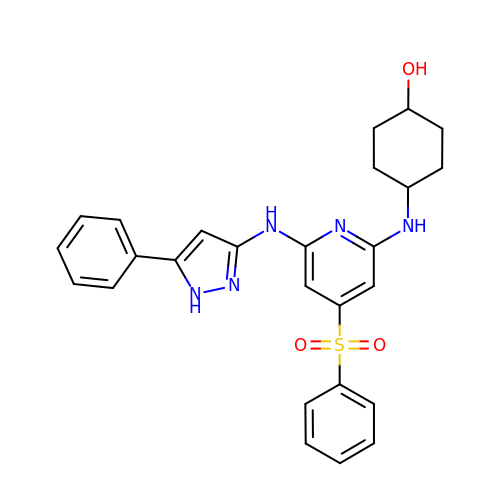trans-4-({6-[(5-phenyl-1H-pyrazol-3-yl)amino]-4-(phenylsulfonyl)pyridin-2-yl}amino)cyclohexanol | C26 H27 N5 O3 S | YIGXUZJWVOKKIO-MXVIHJGJSA-N> AEAGITGTWYNQLGSTFIVTAGADGALT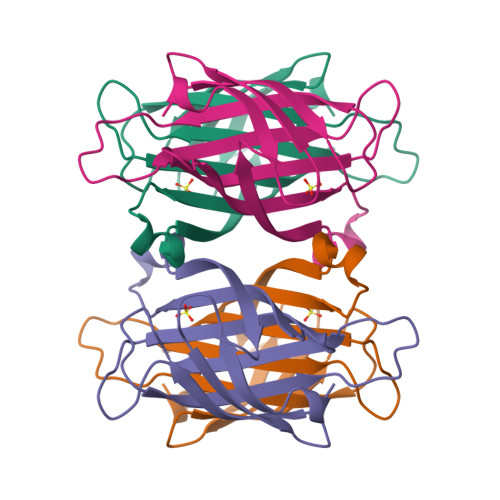GTYESAVGNAESRYVLTGRYDSAPATDGSGTALGWTVAWKNNYRNAHSATTWSGQYVGGAEARINTQWLLTSGTTEANAWKSTLVGHDTFTKVK>[2x]MAGDSEQTLQNHQQPNGGEPFLIGVSGGTASGKSSVCAKIVQLLGQNEVDYRQKQVVILSQDSFYRVLTSEQKAKALKGQFNFDHPDAFDNELILKTLKEITEGKTVQIPVYDFVSHSRKEETVTVYPADVVLFEGILAFYSQEVRDLFQMKLFVDTDADTRLSRRVLRDISERGR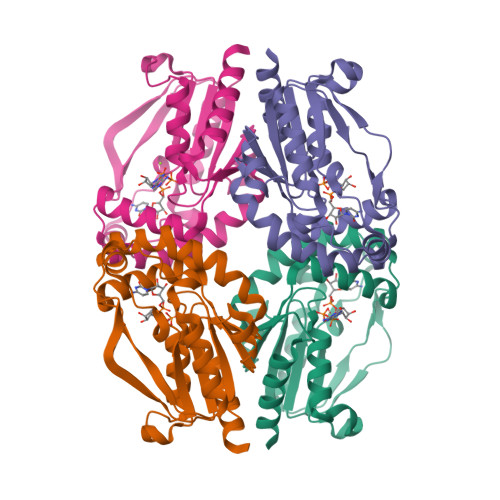DLEQILSQYITFVKPAFEEFCLPTKKYADVIIPRGADNLVAINLIVQHIQDILNGGPSKRQTNGCLNGYTPSRKRQASESSSRPH>VTALSRLGEPPSGHDGNSEVRRIAMKRATVPVLRRVAAVCAAALLVTVGTGGPASATGTRSAICRATTVEVTLGKGTGKMWGELCRPAGSSPDTVVTMVHGATYNHNYWDFPYQPDKYSFRKMLNGAGYATFVVDRLGTGNSTVPPSSELNLTVEARQMHEVVQGLRTGRIGGTGFGKVVLAGYALGSAVTSIEASTFHDVDAVLITALGHYNNPAGTQAIIDNGLSPNDDPVLKDRHHYDDGYATTKPGSRKHVFYADRPMDPGVLATDELTKDANVFTEAADPLVIDPAVSRAIDVPVMFALGDRDPLMCGDGYEDCSSQAALRAQEAPFWTSAPSFDVILVEDAGHGLNL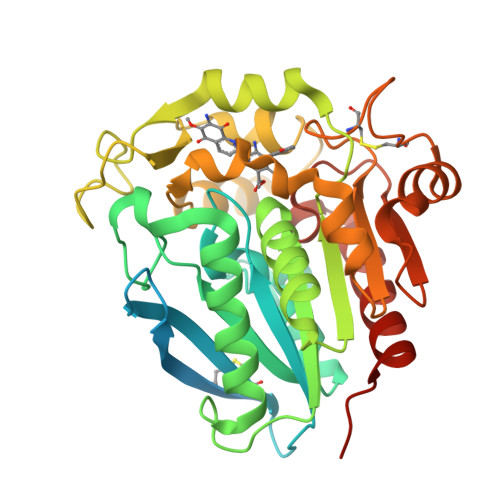VPNTRVYQDASRDWLDRVVGHGLEHHHHHH[7x]>ARKSVLVVRHGERVDQIFGKAWLQQ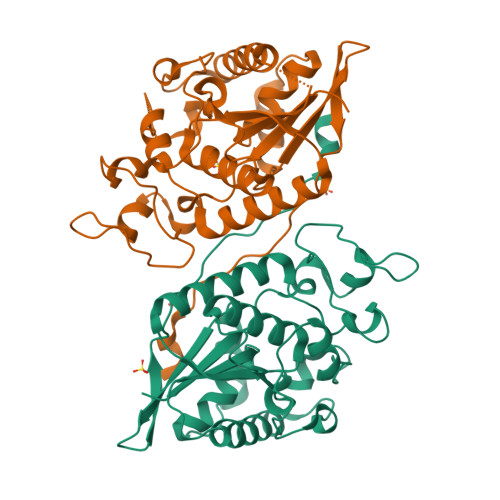CSTPDGKYYRPDLNFPCSLPRRSRGIKDFENDPPLSSCGIFQSRIAGDALLDSGIRISSVFASPALRCVQTAKLILEELKLEKKIKIRVEPGIFEWTKWEAGKTTPTLMSLEELKEANFNIDTDYRPAFPLSALMPAESYQEYMDRCTASMVQIVNTCPQDTGVILIVSHGSTLDSCTRPLLGLPPRECGDFAQLVRKIPSLGMCFCEENKEEGKWELVNPPVKTLTHGANAAFNWRNWI[2x]> MSMLKREDWYDLTRTTNWTPKYVTENELFPEEMSGARGISMEAWEKYDEPYKITYPEYVSIQREKDSGAYSIKAALERDGFVDRADPGWVSTMQLHFGAWALEEYAASTAEARMARFAKAPGNRNMATFGMMDENRHGQIQLYFPYANVKRSRKWDWAHKAIHTNEWAAIAARSFFDDMMMTRDSVAVSIMLTFAFETGFSNMQFLGLAADAAEAGDHTFASLISSIQTDESRHAQQGGPSLKILVENGKKDEAQQMVDVAIWRSWKLFSVLTGPIMDYYTP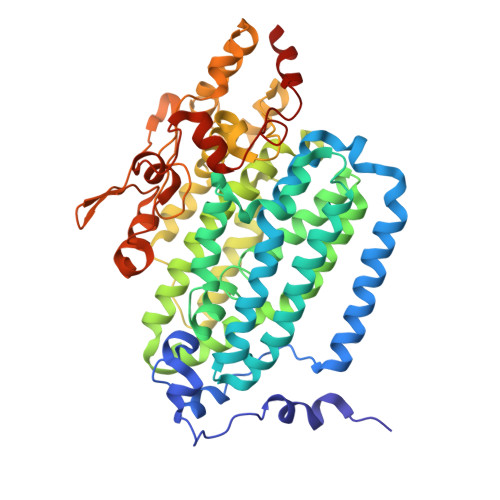LESRNQSFKEFMLEWIVAQFERQLLDLGLDKPWYWDQFMQDLDETHHGMHLGVWYWRPTVWWDPAAGVSPEEREWLEEKYPGWNDTWGQCWDVITDNLVNGKPELTVPETLPTICNMCNLPIAHTPGNKWNVKDYQLEYEGRLYHFGSEADRWCFQIDPERYKNHTNLVDRFLKGEIQPADLAGALMYMSLEPGVMGDDAHDYEWVKAYQKKTNAA5-amino-1,2-dimethylpyridinium | C7 H11 N2 | 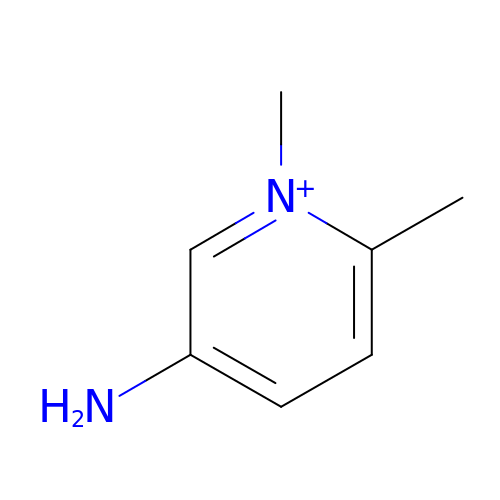FRIAZNRYPWQFFM-UHFFFAOYSA-N> PTHIAIGIYFNPEIAPAPFISLIETNQCAL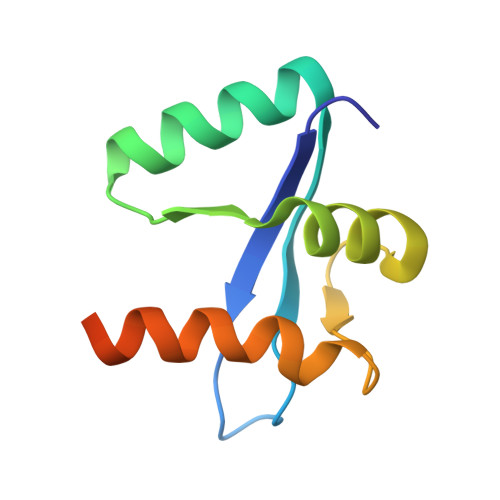AVRKYANEVGIPTVRDVKLARKLYKTHTKYSFVDFEHLDEVLRLIVWLEQVENTHLEHHHHHH The periplasmic chaperone SilF has been identified as part of an Ag(I) detoxification system in Gram-negative bacteria. Biophysical and biochemical analysis of proteins comprising the sil gene cluster has been limited to date, with sequence homology used to infer function and the proposed resistance mechanism, after comparison with the more extensively studied cus and cue systems. Such analysis is consistent with the model that the SilF is a periplasmic metal-binding chaperone capable of binding both Ag(I) and Cu(I) ions and shuttling them to the SilCBA complex to aid metal ion detoxification. The protein has a β-barrel topology composed of five β-stands arranged in the β1-β2-β3-β5-β4-β1, similar to that observed for Cu(I) chaperone CusF. The X-ray crystal structures show that the metal ion–binding site is formed from strictly conserved residues His63, Trp71, Met74, and Met76 located at one end of the β-barrel.

Next, we determined the structure of SilF38-120 using X-ray protein crystallography. Unlike CusF, SilF38-120 has an additional 15 amino acid α-helix positioned between strands β3-β5. In CusF, this is an extended loop with no discernable helical or sheet secondary structural elements. RMSDs derived from the Cα atoms are 0.99 Å for Ag(I)/Apo and 1.09 Å for Cu(I)/Apo. Larger deviations are observed primarily in the metal-binding site, the top of the α-helix, and the final loop that leads into the C terminus. Recalculating RMSDs with these two regions missing reduces the value to 0.68 Å for Ag(I)/Apo and 0.98 Å for Cu(I)/Apo, showing that changes in flexibility is confined to the binding site and these regions. Although we do not see appreciable changes in helix formation from the crystal structures, most likely due to crystal packing forces, both of the solution experimental observations are well supported by the simulations where changes in helicity are clearly over long simulation times between the apo and holo SilF. Together, these show that the capping helix is unstable in the apo-protein and indeed could be unfolded to a degree in solution, as observed for CusF, with metal binding stabilizing the helix by an as-yet undefined allosteric mechanism.

>[3x]RNSLKAVLFGAFSVMFSAGLHAETHQHGDMNAASDASVQQVIRGSGVVKAIDMNSKKITISHEAIPAVGWPAMTMRFTFVNADDAIDAINALKTGNHVDFSFIQQGNISLLKSINVTQS>[2x]VIDPSELTFVQEIGSGQFGLVHLGYWLNKDKVAIKTIREGAMSEEDFIEEAEVMMKLSHPKLVQLYGVCLEQAPICLVFEFMEHGCLSDYLRTQRGLFAAETLLGMCLDVCEGMAYLEEACVIHRDLAARNCLVGENQVIKVSDFGMTRFVLDDQYTSSTGTKFPVKWASPEVFSFSRYSSKSDVWSFGVLMWEVFSEGKIPYENRSNSEVVEDISTGFRLYKPRLASTH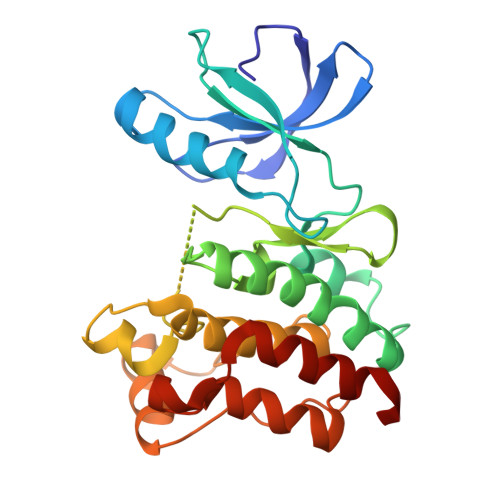VYQIMNHCWKERPEDRPAFSRLLRQLAEIAESGL> GAGUGCC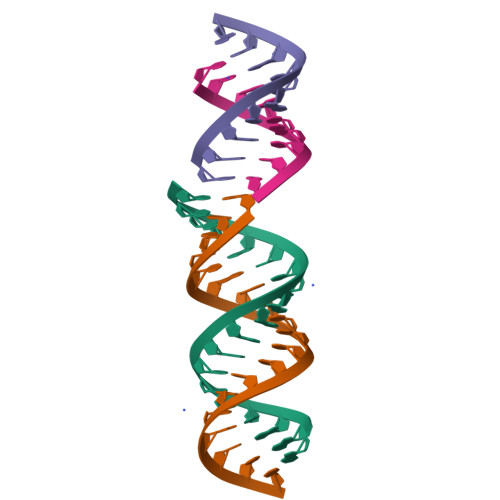AGAAGCUGCCUC;> GAGUGCCAGA;> GAGGCAGUUUCUGGUACUC;> CUGGUACUC>[180x]MTLEQAIERAGTKHGNKGWEAALSAIEMANLFKSLRGTGGSGSSMEIYEGKLTAEGLRFGIVASRFNHALVDRLVE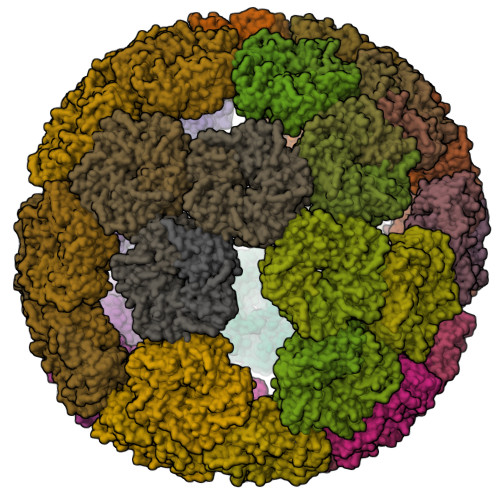GAIDCIVRHGGREEDITLVRVPGSWEIPVAAGELARKEDIDAVIAIGVLIRGATPHFDYIASEVSKGLANLSLELRKPITFGVITAD> QDAHQKMGHGAATPSTAPTGRPLPLPPLVEPDASGVVKLKVQTGRHSFEEGSEAASAGINGAYLGPLVRLKNGETVTLSVENGMDEGTTLHWHGLFVPSILDGGPHNVIAAGEAWKPEVKIQQPASFNWFHPHLHGNTARQAHLGIAGLMVVTDGKDAERGLPEDYGVDDIPLVLQDRRVIEGDKVYEPDIMDLMHGFRGGNLIVNGIVSPEARVPASIVRLRILNGANARNFHVRLSDNRPLLVVASDGGFIGNPEPVERLTISPGERYEVLVDFSKGEATDLLTYGDDSGGDDLHLMRFVVDAALQGKVTKRPDRLDGPDAPDEKLSVKRRSFFFDERMAENMKLMMAKLSADPHAGHNMGNMDMG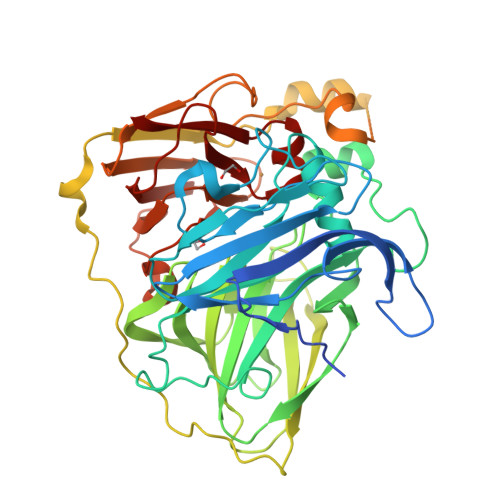SMQSGAMDHDMHGARSSADAGPALEALTSGVEMAIAGKPFDMDRIDVEAKLGSWEIWDLTTKEMPHPFHIHGASFRILSLNGKAPPAHQSGWKDTALIDGKAEILVHFDREAVKSHPFMFHCHVLEHEDVGMMAQFVTV AARSs play an essential role in protein synthesis by charging tRNAs with their cognate amino acids. Similar to other LeuRSs, the C. muris LeuRS contains a predicted editing domain exhibiting highly conserved motifs that are important for the hydrolysis of tRNALeu mischarged with noncognate amino acids, such as isoleucine or norvaline, while excluding cognate Leu-tRNALeu. The structures show the typical seven-β-strand and three-α-helix fold of the LeuRS connective polypeptide domain (CP1), plus archaeon/eukaryote-specific insertions, denoted I1ae, I2ae, I3ae, and I4ae.

Despite predicted flexibility, the three insertions are, in fact, ordered and include well-defined secondary structure elements. Iax3 consists of a β-tongue structure which connects the α-helix (αae1) and the third β-sheet (βae3) of I2ae. Interestingly, Iax3 has a well-defined β-sheet in the apo-structure, whereas all the holo-structures show a significantly different conformation with shifts of up to 8.9 Å. Another difference between the apo- and holo-structures is the position of helices α1 and α2 adjacent to I4ae at the editing site, which needs to open (∼1.5 Å) to accommodate ligands. Overall, the CmLeuRS insertions are 25 to 45 Å distant from the editing site and thus are presumably not directly involved in posttransfer editing, although we cannot exclude this possibility in the context of the full-length protein and tRNA.

>GAMGPQEYTLIKLKIHLIPEFLGSIVKGREVFVVCATLRPETMYGQTNCWILPDGEYDLVLAFDQVIPYDAKTSDGVLCKIFDKYEDTMKECNTVYICSERSAYNMAYQGIVPLIHGREQGVSDKLLPRIVSLGKVYGEQLIGTPLSAPMTPYSLIFILPMFSISMEKGTGIVTSVPSDSPDDYAALRDIKTKPLLREKYSIKDEWILDPLEIIEVPGFGFMTAELLCNQYKIQSQNDSAKLKQAKEEIYKKEFYEGILIRGKYSGMKICDAKELIRESLIKDGYALIYLE[3x];> GAMGPQEYTLIKLKIHLIPEFLGSIVKGREVFVVCATLRPETMYGQTNCWILPDGEYDLVLAFDQVIPYDAKTSEGVLCKIFDKYEDTMKECNTVYICSERSAYNMAYQGIVPLIHGREQGVSDKLLPRIVSLGKVYGEQLIGTPLSAPMTPYSLIFILPMFSISMEKGTGIVTSVPSDSPDDYAALRDIKTKPLLREKYSIKDEWILDPLEIIEVPGFGFMTAELLCNQYKIQSQNDSAKLKQAKEEIYKKEFYEGILIRGKYSGMKICDAKELIRESLIKDGYALIYLE N,N-BIS(4-CHLOROBENZYL)-1H-1,2,3,4-TETRAAZOL-5-AMINE 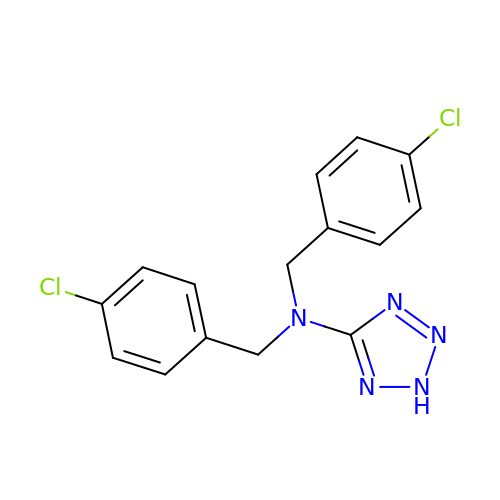| C15 H13 Cl2 N5 | UOUXILZUBDIWQU-UHFFFAOYSA-N> MTTLLQTLLIRTLSEQKDYILLEYFQTILPALEEHFGNTSGLGGSFISHQKHFGTQGYDTEKAKKMAQGFAKKGDQTLAAHILNALLTTWNVMQELEFPLNDIERRLLCLGITLHDYDKHCHAQDMAAPEPDNIQEIINICLELGKRLNFDEFWADWRDYIAEISYLAQNTHGKQHTNLISSNWSNAGYPFTIKERKLDHPLRHLLTFGDVAVHLSSPHDLVSSTMGDRLRDLLNRLGIEKRFVYHHLRDTTGILSNAIHNVILRTVQKLDWKPLLFFAQGVIYFAPQDTEIPERNEIKQIVWQGISQELGKKMSAGDVGFKRDGKGLKVSPQTSELLAAADIVRILPQVISVKVNNAKSPATPKRLEKLELGDAEREKLYEVADLRCDRLAELLGLVQKEIFLLPEPFIEWVLKDLELTSVIMPEETQVQSGGVNYGWYRVAAHYVANHATWDLEEFQEFLQGFGDRLATWA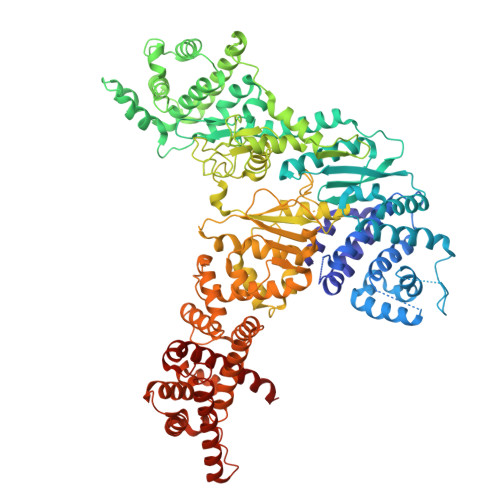EEEGYFAEHQSPTRQIFEDYLDRYLEIQGWESDHQAFIQELENYVNAKTKKSKQPICSLSSGEFPSEDQMDSVVLFKPQQYSNKNPLGGGQIKRGISKIWSLEMLLRQAFWSVPSGKFEDQQPIFIYLYPAYVYAPQVVEAIRELVYGIASVNLWDVRKHWVNNKMDLTSLKSLPWLNEEVEAGTNAQLKYTKEDLPFLATVYTTTREKTDTDAWVKPAFLALLLPYLLGVKAIATRSMVPLYRSDQDFRESIHLDGVAGFWSLLGIPTDLRVEDITPALNKLLAIYTLHLAARSSPPKARWQDLPKTVQEVMTDVLNVFALAEQGLRREKRDRPYESEVTEYWQFAELFSQGNIVMTEKLKLTKRLVEEYRRFYQVELSKKPSTHAILLPLSKALEQILSVPDDWDEEELILQGSGQLQAALDRQEVYTRPIIKDKSVAYETRQLQELEAIQIFMTTCVRDLFGEMCKGDRAILQEQRNRIKSGAEFAYRLLALEAQQNQN> GSMFLQRPKPYSDESLESFFIRVANKNGYGDVHRFLEATKRFLQDIDHNGYQTFPTDITRINPYSAKNSSSARTASFLKLAQLTFNEPPELLGLAINRTNMKYSPSTSAVVRGAEVFPRSLLRTHSIPCCPLCLRENGYASYLWHFQGY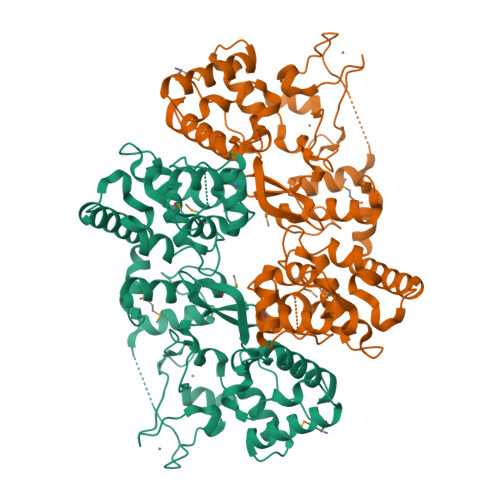EYCHSHNVPLITTCSCGKEFDYRVSGLKGICCKCKEPITLTSRENGHEAACTVSNWLAGHESKPLPNLPKSYRWGLVHWWMGIKDSEFDHFSFVQFFSNWPRSFHSIIEDEVEFNLEHAVVSTSELRLKDLLGRLFFGSIRLPERNLQHNIILGELLCYLENRLWQDKGLIANLKMNALEATVMLNCSLDQIASMVEQRILKPNRKSKPNSPLDVTDYLFHFGDIFCLWLAEFQSDEFNRSFYVSRW> MGSDKIHHHHHHMSKKQKSKYIVIFGCGRLGSLIANLASSSGHSVVVVDKNEYAFHRLNSEFSGFTVVGDAAEFETLKECGMEKADMVFAF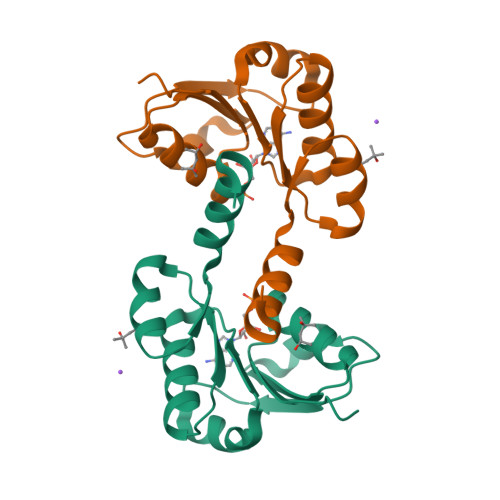TNDDSTNFFISMNARYMFNVENVIARVYDPEKIKIFEENGIKTICPAVLMIEKVKEFIIGSEED>MHHHHHHSNLLTVHQNLPALPVDATSDEVRKNLMDMFRDRQAFSEHTWKMLLSVCRSWAAWCKLNNRKWFPAEPEDVRDYLLYLQARGLAVKTIQQHLGQLNMLHRRSGLPRPSDSNAVSLVMRRIRKENVDAGERAKQALAFERTDFDQVRSLMENSDRCQDIRNLAFLGIAYNTLLRAAEIARIRVKDISRTDGGRMLIHIGRTKTLVSTAGVEKALSLGVTKLVERWISVSGVADDPNNYLFCRVRKNGVAAPSATSQLSLSALHGIFGATHRLIYGAKDDSGQRYLAWSGHSARV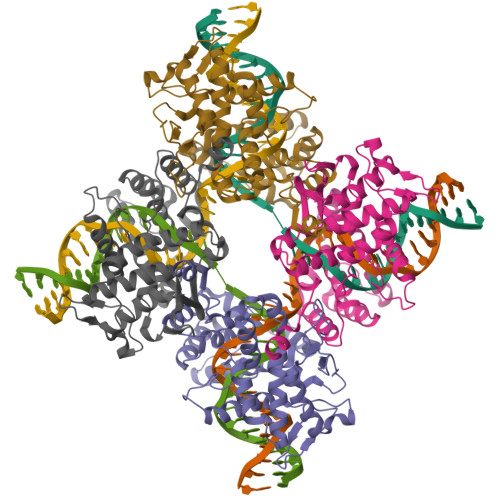GAARDMARAGVSIPEIMQAGGWTNVNIVMNYIRNLDSETGAMVRLLEDGD[2x]> MSTKKKPLTQEQLEDARRLKAIYEKKKNELGLSQESVADKMGMGQSGVGALFNG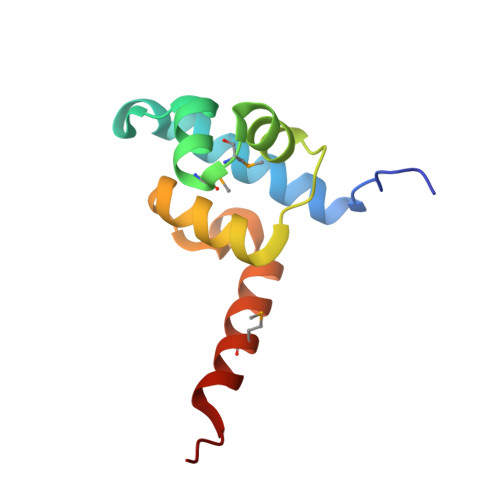INALNAYNAALLAKILKVSVEEFSPSIAREIYEMYEAVHHHHHH>MDVVSLDKPFMYFEEIDNELDYEPESANEVAKKLPYQGQLKLLLGELFFLSKLQRHGILDGATVVYIGSAPGTHIRYLRDHFYNLGVIIKWMLIDGRHHDPILNGLRDVTLVTRFV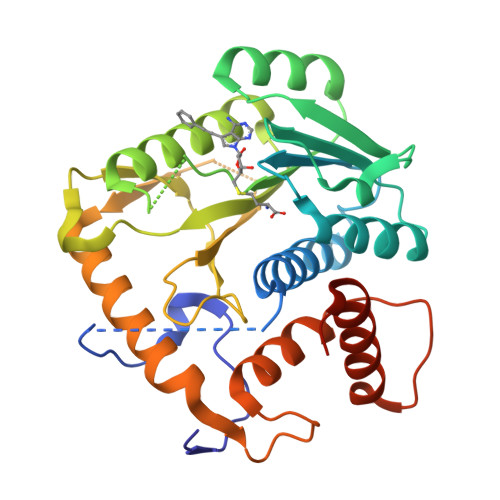DEEYLRSIKKQLHPSKIILISDVRSKRGGNEPSTADLLSNYALQNVMISILNPVASSLKWRCPFPDQWIKDFYIPHGNKMLQPFAPSYSAEMRLLSIYTGENMRLTRVTKSDAVNYEKKMYYLNKIVRNKVVINFDYPNQEYDYFHMYFMLRTVYCNKTFPTTKAKILFLQQSIFRFLNIPTTSTEKVSHE[2x]>[2x]MRGLSRRVQAMKPSATVAVNAKALELRRQGVDLVALTAGEPDFDTPEHVKEAARRALAQGKTKYAPPAGIPELREALAEKFRRENGLSVTPEETIVTVGGKQALFNLFQAILDPGDEVIVLSPYWVSYPEMVRFAGGVVVEVETLPEEGFVPDPERVRRAIT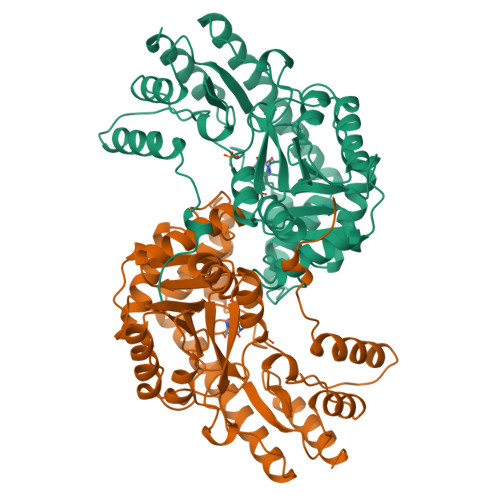PRTKALVVNSPNNPTGAVYPKEVLEALARLAVEHDFYLVSDEIYEHLLYEGEHFSPGRVAPEHTLTVNGAAKAFAMTGWRIGYACGPKEVIKAMASVSSQSTTSPDTIAQWATLEALTNQEASRAFVEMAREAYRRRRDLLLEGLTALGLKAVRPSGAFYVLMDTSPIAPDEVRAAERLLEAGVAVVPGTDFAAFGHVRLSYATSEENLRKALERFARVL> SEFENPLKQLLAEEQWEFEVTAFYRGRQVFQQTLFCPGGLRLVGSTADMTLPWQPVTLPDPEGFLTDK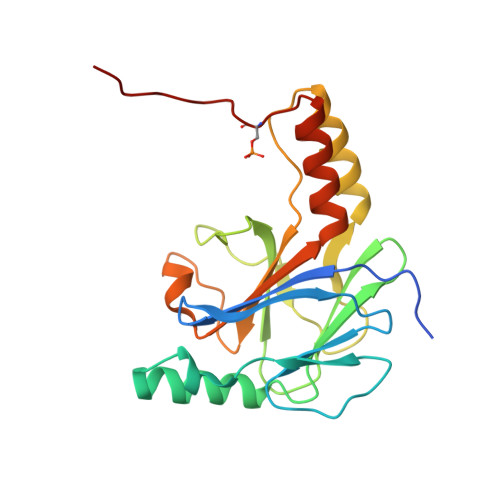LVKEYVGQVLKGLGNGLALWQAGQCLWAQRLGHSHAFWALGEELLPDSGRGPDGEVHKDKDGAVFDLRPFVADLIAFMEGSGHSPRYTLWFCMGEMWPQDQPWVKRLVMVKVVPTCLKELLEMAREGGASSLKTVDLHISNS>MDKKT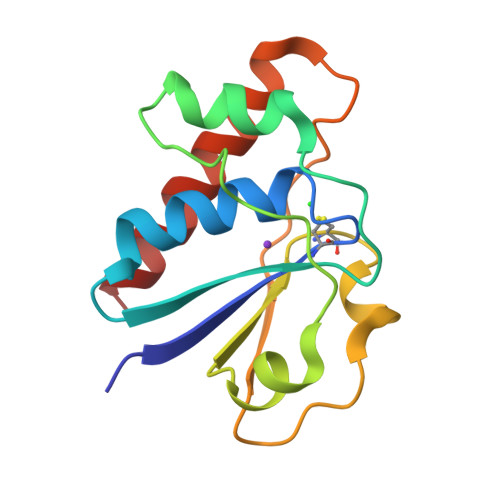IYFICTGNSCRSQMAEGWGKEILGEGWNVYSAGIETHGVNPKAIEAMKEVDIDISNHTSDLIDNDILKQSDLVVTLCSDADNNLPILPPNVKKEHWGFDDPAGKEWSEFQRVRDEIKLAIEKFKLR[2x]3-Phosphoglycerate dehydrogenase (PHGDH) catalyzes the first step in the de novo serine synthesis pathway, i.e. the NAD+-dependent conversion of 3-phosphoglycerate (3-PG) to phosphohydroxypyruvate (PHP). PHGDH diverts the glycolytic flux towards producing serine, which in turn is metabolized and incorporated into a variety of biomolecules including glycine, thereby providing a major source of one-carbon units for the synthesis of purine and pyrimidine nucleotides. Type I enzymes contain two additional regulatory domains, the ACT (aspartate kinase-chorismate mutase-tyrA prephenate dehydrogenase) and ASB (allosteric substrate binding) domains.

Here, in order to better understand the substrate and catalytic promiscuity of human PHGDH and to identify other potential roles of PHGDH that might be relevant in diseases, such as cancer, we have developed and applied functional and binding assays for PHGDH, and have solved structures for the catalytic domain in complex with its cofactor NAD+ both alone and together with the substrate analogue L-tartrate. In agreement with the deposited structure of sPHGDH, two molecules were present in the crystallographic asymmetric unit (ASU). However, while both molecules had NAD+ bound to the cofactor sites, L-tartrate was only present in one molecule, allowing comparison of substrate-bound and unbound states. In both domains, NAD+ was bound in the same way, forming various hydrogen bonds with the enzyme. The substrate analogue, L-tartrate, interacted with both the lid and the core domain of sPHGDH, through a network of hydrogen bonds. L-Tartrate formed hydrogen bonds to R235, H282 and A285 of the core domain and to R53, S54, R74, T77 and Q291 of the lid domain. In the absence of L-tartrate, the lid domain, which otherwise closed over the substrate-binding site, underwent a rigid domain movement. In order to characterize the movement, the two molecules in the ASU were compared using the DynDom webserver. This analysis suggested three structural sub domains: a fixed core domain (aa 100-287), a mobile lid domain (aa 9-93 and aa 289-301) and a hinge domain (aa 94-99 and aa 302). Interestingly, superposition of the two conformations with and without bound L-tartrate showed that the lid domain had rotated by 29° upon substrate binding. Comparison of the two molecules showed that in the presence of L-tartrate a movement of the lid domain towards a more closed substrate pocket had occurred, consistent with the hypothesis that the substrate binds after the cofactor.

>[2x]AKVLISDSLDPCCRKILQDGGLQVVEKQNLSKEELIAELQDCEGLIVRSATKVTADVINAAEKLQVVGRAGTGVDNVDLEAATRKGILVMNTPNGNSLSAAELTCGMIMCLARQIPQATASMKDGKWERKKFMGTELNGKTLGILGLGRIGREVATRMQSFGMKTIGYDPIISPEVSASFGVQQLPLEEIWPLCDFITVHTPLLPSTTGLLNDNTFAQCKKGVRVVNCARGGIVDEGALLRALQSGQCAGAALDVFTEEPPRDRALVDHENVISCPHLGASTKEAQSRCGEEIAVQFVDM>[2x]SWNKKNEEKEDFGIIVILWKQVTVKEDGKVPLEPFLTAAKEVLRVVDAFGSGFRIVKNDIAGNIKKLY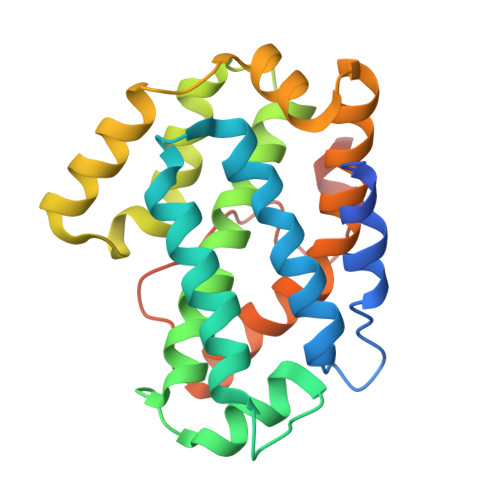RANQTVHAETLQELIIAENSPDGLATVALLWLKRAFQFIASFLRRLVVTDKSLEQCVTEAYNCTLRPCHSAVIQKVFWGGVKLAPSRERFYRKLHPDLNIAKAKIEEFLIELHDPLCCIVQFFFQRELEDQCWGDEVYQRKDSSEWLKVSCEQDSV>RSQENSFTINSVDMKSLPDWTVQNGKNLTLQCFADVSTTSHVKPQHQMLFYKDDVLFYNISSMKSTESYFIPEVRIYDSGTYKCTVIVNNKEKTTAEYQLLVEGVPSPRVTLDKKEAIQGGIVRVNCSVPEEKAPIHFTIEKLELNEKMVKLKRE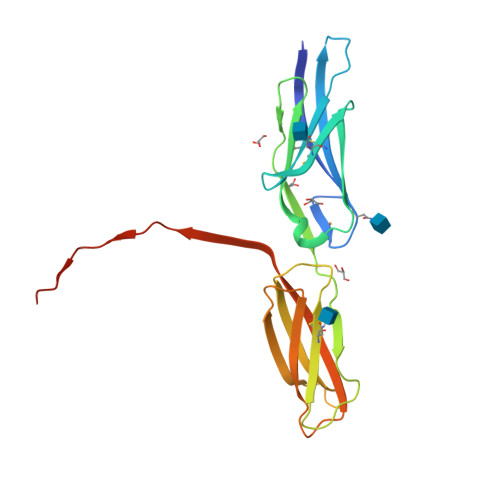KNSRDQNFVILEFPVEEQDRVLSFRCQARIISGIHMQTSESTKSELVTVSRENLYFQ[2x]> SNAMVSTIGIVSLSSGIIGEDFVKHEVDLGIQRLKDLGLNPIFLPHSLKGLDFIKDHPEARAED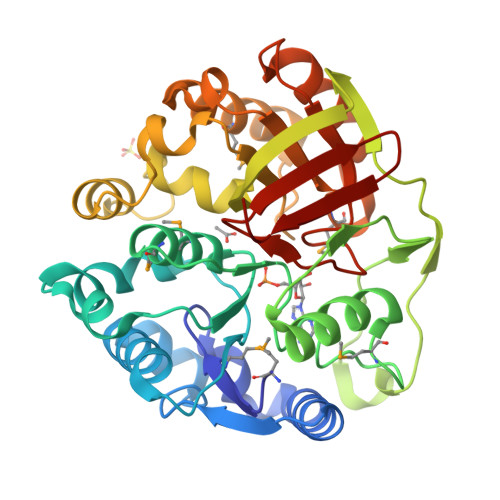LIHAFSDDSIDMILCAIGGDDTYRLLPYLFENDQLQKVIKQKIFLGFSDTTMNHLMLHKLGIKTFYGQSFLADICELDKEMLAYSLHYFKELIETGRISEIRPSDVWYEERTDFSPTALGTPRVSHTNTGFDLLQGSAQFEGKILGGCLESLYDIFDNSRYADSTELCQKYKLFPDLSDWEGKILLLETSEEKPKPEDFKKMLLTLKDTGIFAVINGLLVGKPMDETFHDDYKEALLDIIDSNIPIVYNLNVGHATPRAIVPFGVHAHVDAQEQVILFDYNK>[2x]MIRLIFLDIDKTL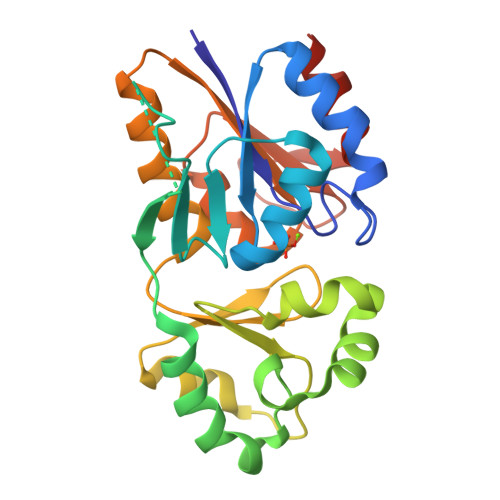IPGYEPDPAKPIIEELKDMGFEIIFNSSKTRAEQEYYRKELEVETPFISENGSAIFIPKGYFPFDVKGKEVGNYIVIELGIRVEKIREELKKLENIYGLKYYGNSTKEEIEKFTGMPPELVPLAMEREYSETIFEWSRDGWEEVLVEGGFKVTMGSRFYTVHGNSDKGKAAKILLDFYKRLGQIESYAVGDSYNDFPMFEVVDKVFIVGSLKHKKAQNVSSIIDVLEVIKHHHHHH> GSHMGHIIDISKWNGDINWSIAKQHIDFIIARVQDGSNYVDPLYKGYVQAMKQHGIPFGNYAFCRFVSIADAKKEAQDFWNRGDKSATVWVADVEVK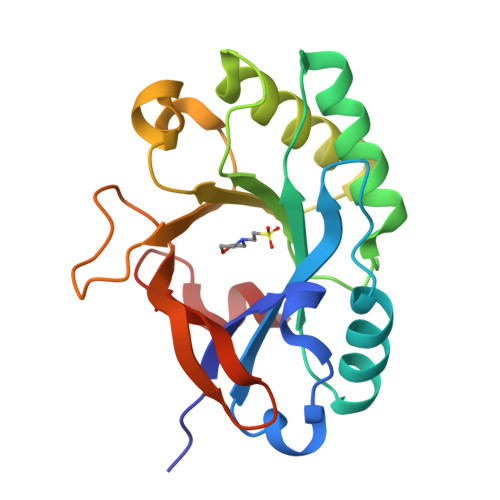TMNDMRAGTQAFIDELYRLGAKKVGLYVGHHMYTPFGMANVKSDFVWIPRYGGNKPAYPCDIWQYTETGNVPGIGKCDLNSLIGNKSLSWFTESA> GHMSGRGKKPTRTLVMTSMPSEKQNVVIQVVDKLKGFSIAPDVCETTTHVLSGKPLRTLNVLLGIARGCWVLSYDWVLWSLELGHWISEEPFELSHHFPAAPLCRSECHLSAGPYRGTLFADQPVMFVSPASSPPVAKLCELVHLCGGRVSQVPRQASIVIGPYSGKKKATVKYLSEKWVL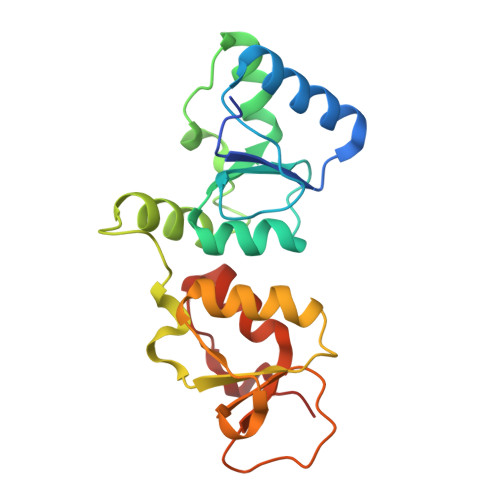DSITQHKVCAPENYLLSQ>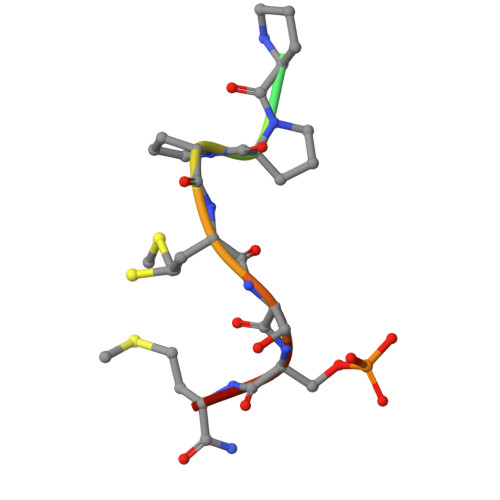 XFMPPPMSSMX> DTKTVQNGYFEDAAVKDRTLSDYAGNWQSVYPFLEDGTFDQVFDYKAKLTGKMTQAEYKAYYTKGYQTDVTKINITDNTMEFVQGGQSKKYTYKYVGKKILTYKKGNRG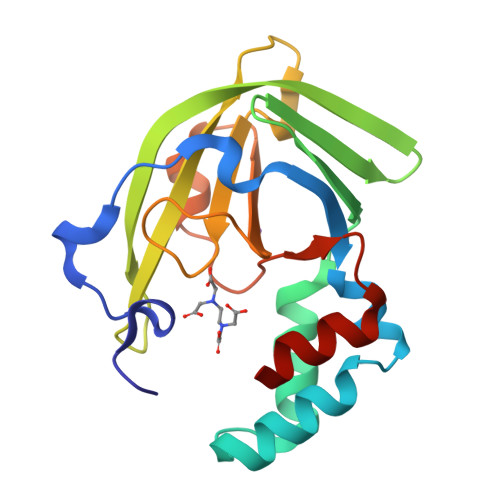VRFLFEATDADAGQFKYVQFSDHNIAPVKAEHFHIFFGGTSQETLFEEMDNWPTYYPDNLSGQEIAQEMLAH> MASHTADADAKPDSDSQKLLNVLPVSLRLRTRPWWFPIQEVSNPLVLYMEAWVAERVIGTDQAEISEIEWMCQALLTVDSVNSGNLAEITIFGQPSAQTRMKNILLNMAAWH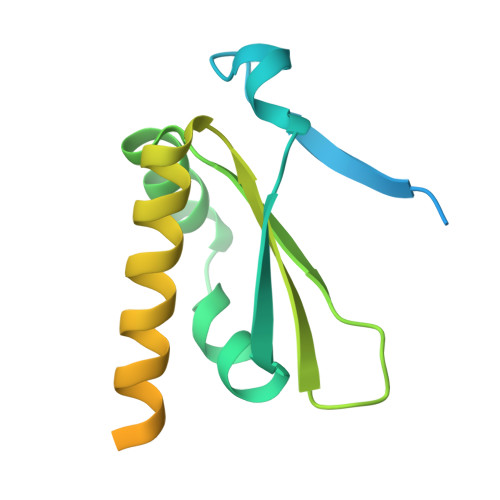KENELQRAVKVKEVEEFLKIRASSILSKLSKKGLKLAGFPLPLEGRETQMES>[2x]MKNKVQLITYADRLGDGTIKSMTDILRTRFDGVYDGVHILPFFTPFDGADAGFDPIDHTKVDERLGSWDDVAELSKTHNIMVDAIVNHMSWE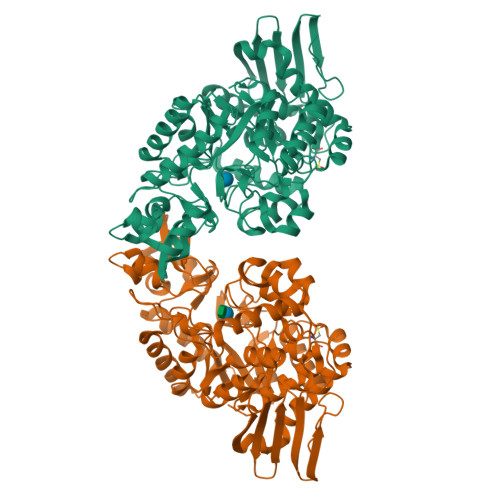SKQFQDVLAKGEESEYYPMFLTMSSVFPNGATEEDLAGIYRPRPGLPFTHYKFAGKTRLVWVSFTPQQVDIDTDSDKGWEYLMSIFDQMAASHVSYIRLDAVGYGAKEAGTSCFMTPKTFKLISRLREEGVKRGLEILIQVHSYYKKQVEIASKVDRVYDFALPPLLLHALSTGHVEPVAHWTDIRPNNAVTVLDTHDGIGVIDIGSDQLDRSLKGLVPDEDVDNLVNTIHANTHGESQAATGAAASNLDLYQVNSTYYSALGCNDQHYIAARAVQFFLPGVPQVYYVGALAGKNDMELLRKTNNGRDINRHYYSTAEIDENLKRPVVKALNALAKFRNELDAFDGTFSYTTDDDTSISFTWRGETSQATLTFEPKRGLGVDNTTPVAMLEWEDSAGDHRSDDLIANPPVVA> MSQEIRQNEKISYRIEGPFFIIHLINPDNLNALEGEDYIYLGELLELADRNRDVYFTIIQSSGRFFSSGADFKGIAKAQGDDTNKYPSETSKWVSNFVARNVYVTDAFIKHSKVLICCLNGPAIGLSAALVALCDIVYSINDKVYLLYPFANLGLITEGGTTVSLPLKFGTNTTYECLMFNKPFKYDIMCENGFISKNFNMPSSNAEAFNAKVLEELRE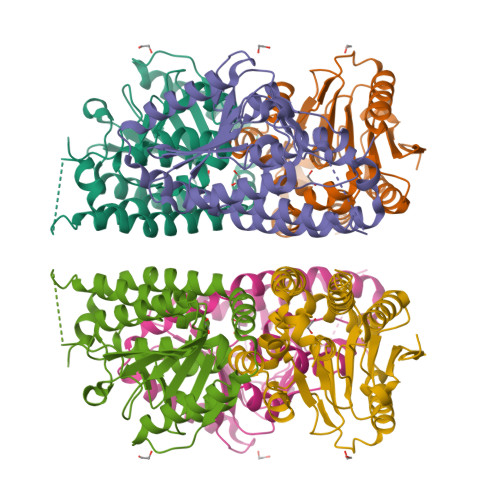KVKGLYLPSCLGMKKLLKSNHIDAFNKANSVEVNESLKYWVDGEPLKRFRQLGSKQRKHRL> GEHIPGTLRFRLSPAARNILEKHSLDASQGTATGPRGIFTKEDALKLVQLKQTGKILE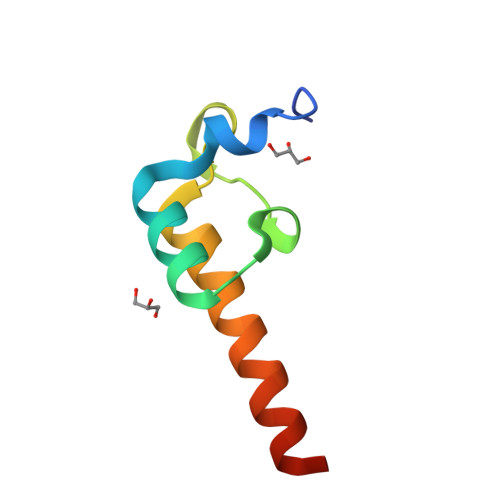HHHHHH> MVQ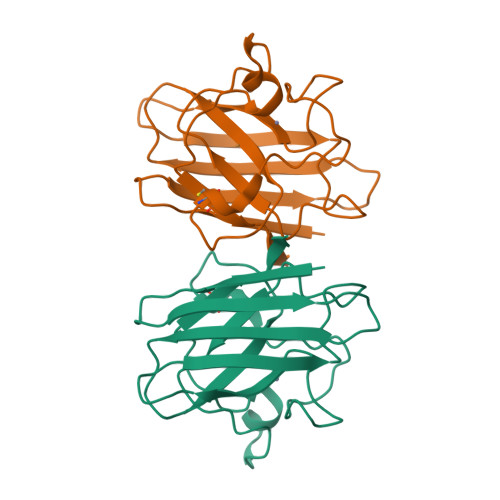AVAVLKGDAGVSGVVKFEQASESEPTTVSYEIAGNSPNAERGFCIHEFGDATNGCVSAGPHFNPFKKTHGAPTDEVRHVGDMGNVKTDENGVAKGSFKDSLIKLIGPTSVVGRSVVIHAGQDDLGKGDTEESLKTGNAGPRPACGVIGLTN> GKSKAELQSEERKRIDELIESGKEEGMKIDLIDGKGRGVI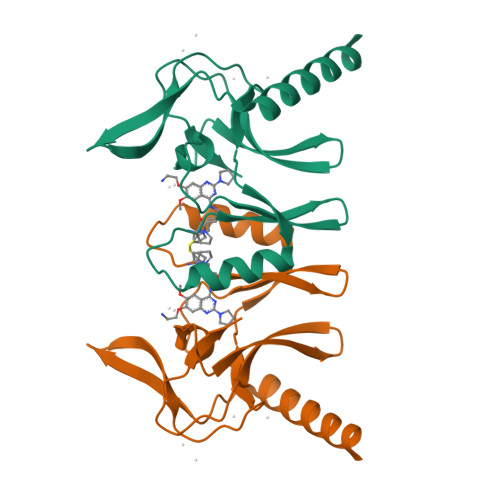ATKQFSRGDFVVEYHGDLIEITDAKKREALYAQDPSTGCYMYYFQYLSKTYCVDATRETNRLGRLINHSKSGNCQTKLHDIDGVPHLILIASRDIAAGEELLYDYGDR> MSLRVRIAVIGKLDGFIKEGIKHYEKFLRRFCKPEVLEIKRVHRGSIEEIVRKETEDLTNRILPGSFVMVMDKRGEEV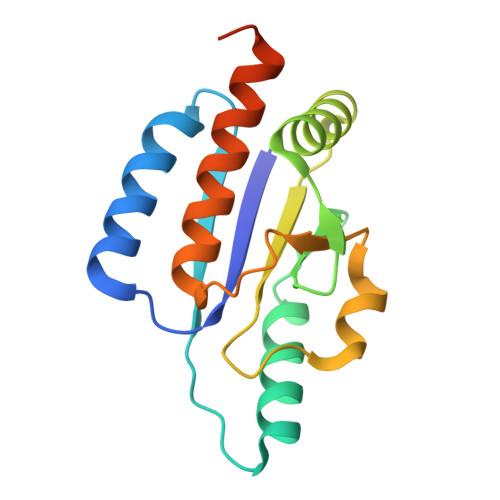SSEEFADFLKDLEMKGKDITILIGGPYGLNEEIFAKAHRVFSLSKMTFTHGMTVLIVLEQIFRAFKIIHGENYHYEGGSHHHHHH4-[(1R)-1-[1-(4-chlorophenyl)-1,2,3-triazol-4-yl]ethoxy]-1-oxidanyl-quinoline | C19 H15 Cl N4 O2 | 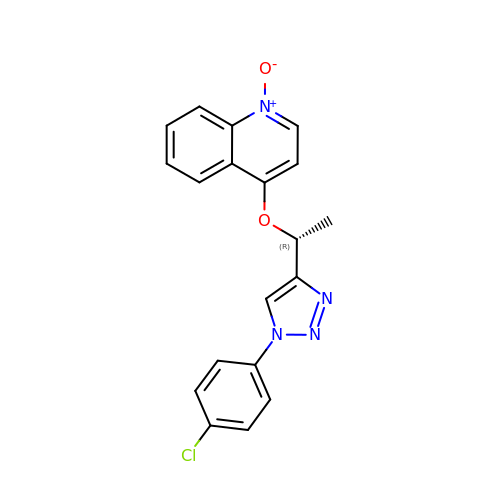SVKHERCOWKMPQO-CYBMUJFWSA-N> GHMNIESTLNSVASVKDLANEASKYEIILQKGINQVGLKQYTQVVHKLDDMLEDIQSGQANREENSEFHGILTHLEQLIKRSEAQLRVYFISILNSIKPFDPQINITKKMPFPYYEDQQLGALSWILDYFHGNSEGSIIQDILVGERSKLILKCMAFLEPFAKEISTAKNAPYEKGSSGMNSYTEALLGFIANEKSLVDDLYSQYTESKPHVLSQILSPLISAYAKLFGANLKIVRSNLENFGFFSFELVESINDVKKSLRGKELQNYNLLQDCTQEVRQVTQSLFRDAIDRIIKKANSISTIPSNNGVTEATVDTMSRLRKFSEYKNGCLGAMDNITRENWLPS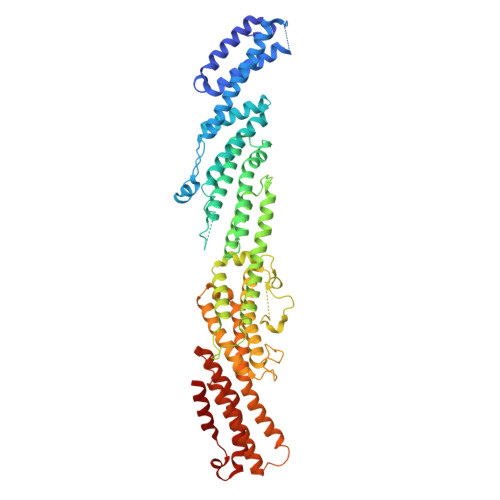NYKEKEYTLQNEALNWEDHNVLLSCFISDCIDTLAVNLERKAQIALMPNQEPDVANPNSSKNKHKQRIGFFILMNLTLVEQIVEKSELNLMLAGEGHSRLERLKKRYISYMVSDWRDLTANLMDSVFIDSSGKKSKDKEQIKEKFRKFNEGFEDLVSKTKQYKLSDPSLKVTLKSEIISLVMPMYERFYSRYKDSFKNPRKHIKYTPDELTTVLNQLVR> EEVRQFRRLFAQLAGDDMEVSATELMNILNKVVTRHPDLKTDGFGIDTCRSMVAVMDSDTTGKLGFEEFKYLWNNIKKWQAIYKQFDVDRSGTIGSSELPGAFEAAGFHLNEHLYSMI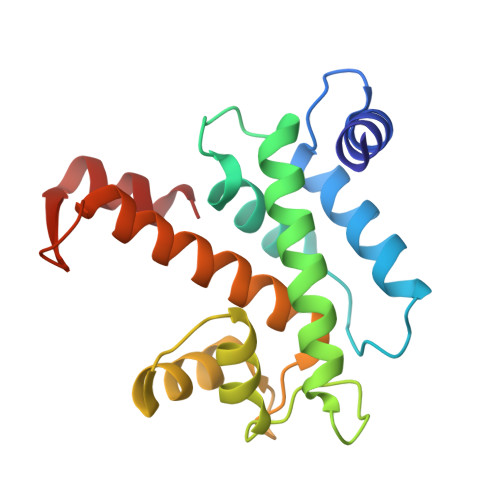IRRYSDEGGNMDFDNFISCLVRLDAMFRAFKSLDKDGTGQIQVNIQEWLQLTMYS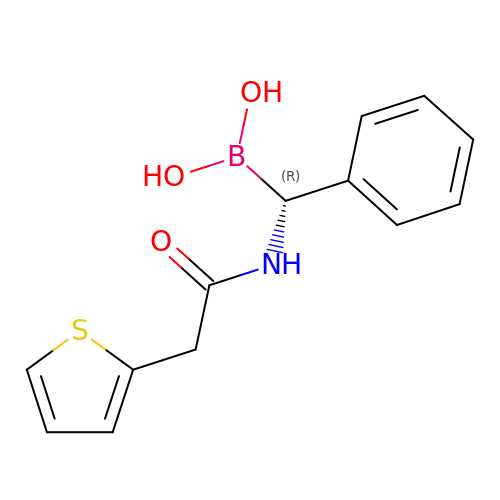(1R)-1-(2-THIENYLACETYLAMINO)-1-PHENYLMETHYLBORONIC ACID | C13 H14 B N O3 S | LGJCDEZMANATFA-ZDUSSCGKSA-N3-(3,5-dimethyl-1,2-oxazol-4-yl)-5-[(phenylsulfonyl)amino]benzoic acid 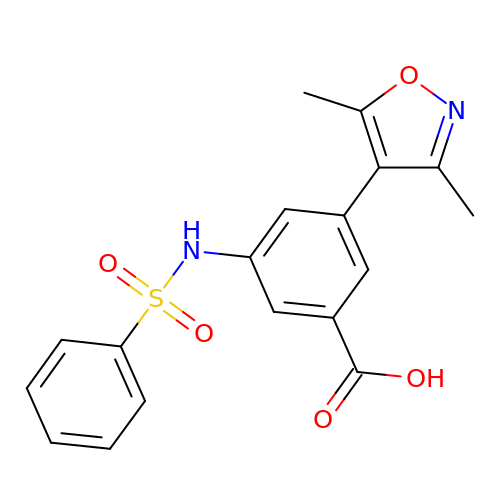| C18 H16 N2 O5 S | FFWKFJNEMDSJKS-UHFFFAOYSA-N>[2x]MSVYGLQRLYIAGAHADATSGKTFDTFDPATGELLARVQQASADDVDRAVASAREGQREWAAMTAMQRSRILRRAVELLRERNDALAELEMRDTGKPIAETRAVDIVTGADVIEYYAGLATA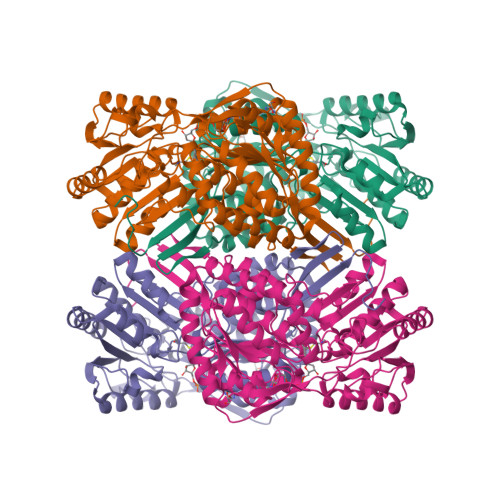IEGLQVPLRPESFVYTRREPLGVCAGIGAWNYPIQIACWKSAPALAAGNAMIFKPSEVTPLSALKLAEIYTEAGVPAGVFNVVQGDGSVGALLSAHPGIAKVSFTGGVETGKKVMSLAGASSLKEVTMELGGKSPLIVFDDADLDRAADIAVTANFFSAGQVCTNGTRVFVQQAVKDAFVERVLARVARIRVGKPSDSDTNFGPLASAAQLDKVLGYIDSGKAEGAKLLAGGARLVNDHFASGQYVAPTVFGDCRDDMRIVREEIFGPVMSILSFETEDEAIARANATDYGLAAGVVTENLSRAHRAIHRLEAGICWINTWGESPAEMPVGGYKQSGVGRENGITTLEHYTRIKSVQVELGRYQPVFGHHHHHH>[2x]GNKWNTTLPGGNMQFQGVIIAETCRIEAGDKQMTVNMGQISSNRFHAVGEDSAPVPFVIHLRECSTVVSERVGVAFHGVADGKNPDVLSVGEGPGIATNIGVALFDDEGNLVPINRPPANWKRLYSGSTSLHFIAKYRATGRRVTGGIANAQAWFSLTYQ;> MGVALGATRVIYPAGQKQEQLAVTNNDENSTYLIQSWVENADGVKDGRFIVTPPLFAMKGKKENTLRILDATNNQLPQDRESLFWMNVKAIPSMDKSKLTENTLQLAIISRIKLYYRPAKLALPPDQAAEKLRFRRSANSLTLINPTPYYLTVTELNAGTRVLENALVPPMGESTVKLPSDAGSNITYRTINDYGALTPKMTGVMEHHHHHH;> DLYFNPRFLADDPQAVADLSRFENGQELPPGTYRVDIYLNNGYMATRDVTFNTGDSEQGIVPCLTRAQLASMGLNTASVAGMNLLADDACVPLTTMVQDATAHLDVGQQRLNLTIPQAFMSNRARGYIPPELWDPGINAGLLNYNFSGNSVQNRIGGNSHYAYLNLQSGLNIGAWRLRDNTTWSYNSSDRSSGSKNKWQHINTWLERDIIPLRSRLTLGDGYTQGDIFDGINFRGAQLASDDNMLPDSQRGFAPVIHGIARGTAQVTIKQNGYDIYNSTVPPGPFTINDIYAAGNSGDLQVTIKEADGSTQIFTVPYSSVPLLQREGHTRYSITAGEYRSGNAQQEKPRFFQSTLLHGLPAGWTIYGGTQLADRYRAFNFGIGKNMGALGALSVDMTQANSTLPDDSQHDGQSVRFLYNKSLNESGTNIQLVGYRYSTSGYFNFADTTYSRMNGYNIETQDGVIQVKPKFTDYYNLAYNKRGKLQLTVTQQLGRTSTLYLSGSHQTYWGTSNVDEQFQAGLNTAFEDINWTLSYSLTKNAWQKGRDQMLALNVNIPFSHWLRSDSKSQWRHASASYSMSHDLNGRMTNLAGVYGTLLEDNNLSYSVQTGYAGGGDGNSGSTGYATLNYRGGYGNANIGYSHSDDIKQLYYGVSGGVLAHANGVTLGQPLNDTVVLVKAPGAKDAKVENQTGVRTDWRGYAVLPYATEYRENRVALDTNTLADNVDLDNAVANVVPTRGAIVRAEFKARVGIKLLMTLTHNNKPLPFGAMVTSESSQSSGIVADNGQVYLSGMPLAGKVQVKWGEEENAHCVANYQLPPESQQQLLTQLSAECRLVPRGSWSHPQFEK

Uropathogenic Escherichia coli strains use filamentous type 1 pili to adhere to and invade uroepithelial cells. The pilus consists of a flexible tip fibrillum, formed by the adhesin FimH and the subunits FimG and FimF. The pilus rod is a helical assembly of up to 3000 copies of the main subunit FimA, terminated by a single copy of the subunit FimI that anchors the rod to the assembly platform FimD in the outer membrane. The assembly platform FimD in the outer membrane of uropathogenic E. coli is the catalyst of type 1 pilus assembly.

To explore the structural implications of FimI-mediated termination of pilus assembly, we performed a FimD-catalyzed assembly reaction of pilus rods in vitro similar to the one for the FimDHGFAnC complex, except that excess FimICHis was also added at the end of the reaction. Since a ten-fold excess of FimICHis over FimD was used to ensure saturation with FimI, we also observed non-physiological states in 3D classification, such as complexes lacking pilus rods due to premature FimI incorporation after FimF, or complexes containing two terminal FimI subunits (FimDHGFAnI2CHis complex, maps XVII and XVIII). Given the low FimI concentrations in the periplasm (FimA:FimI ratio ≥100:1), we focused our analysis on physiological pilus complexes with a single terminal FimI subunit capped by FimCHis.> MTALFLHILWSISYIIINILYIFLSLLLSNNNEKIKQYNSNYFIKILLVLFYNKNLSFYKNLLSEDEISKIEFERLKNYPTLVLIHSNLNKLEKRNKIINSFINFKTKYRFYKFISTNFNLQTIIKNCNDKIIFSTLLYIVNLNYSFFYKTIKNTDLIVYLLANKFSILNDNIIVSKFNISKFNDYIKYINNTNSIDTYLENQIILGLNNNTNSNITKNINTKLLNSYSNLKNLVNITNNTFYLKKINDNYNTVINSEFLTYLKSNYKISFSASNIVKYLSDKSVNNSVILYLRKNKIFNKSRYSRNRQTYRTGAYWCLYVNIIAVVAFYFWFYKFTMNFGYLWWLLYSLILSFFFSRALKHRFYNPLNVMTEFKNGFMWFIIILINIFKPLLKLLENNYINLYNHLVIKYYQSFICNTLINKKKLEFNYILSS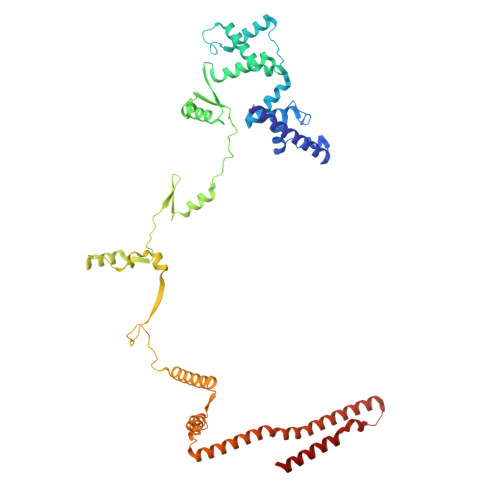FKFIKELNNIIIISLNKLF> TVENFLGRSACVYMEEYKTTDNDVNKKFVAWPINTKQMVQMRRKLEMFTYLRFDMEVTFVITSRQDPGTTLAQDMPVLTHQIMYVPPGGPIPAKVDDYAWQTSTNPSIFWTEGNAPARMSIPFISIGNAYSNFYDGWSNFDQRGSYGYNT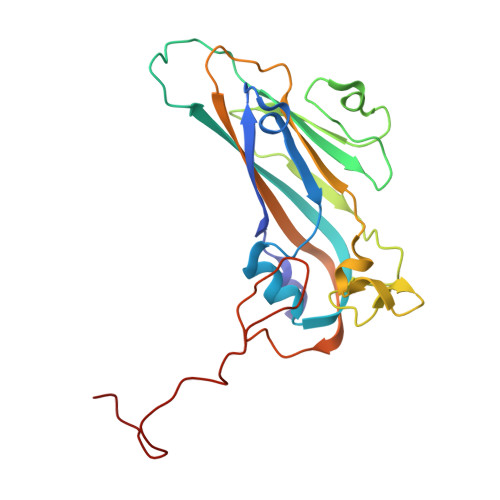LNNLGHIYVRHVSGSSPHPITSTIRVYFKPKHTRAWVPRPPRLCQYKKAFSVDFTPTPITDTRKDINTVTTV>[2x]MASAAKAGDILLSHSFEEGTTQ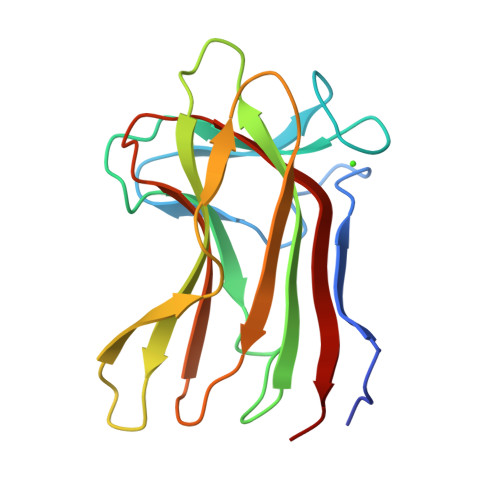GWTARGGVKVDVTAEQAYQGKQSLQTTGRTEAWNGPSLSLTDVVHKNEVVEISGYVKLVAGSAPADLKFTVERRDGNGDTQYDQVNAAEQVTDQKWVKLQGQYSYEQGSSLLLYLESTDAKAAYLLDEFQIRLVKAA> MQKIDEKLQLMNTIAKIYRGSIKEFNNRLGKLMNLSYLDFSILKATSEEPRSMVYLANRYFVTQSAITAAVDKLEAKGLVRRIRDSKDRRIVIVEITPKGRQV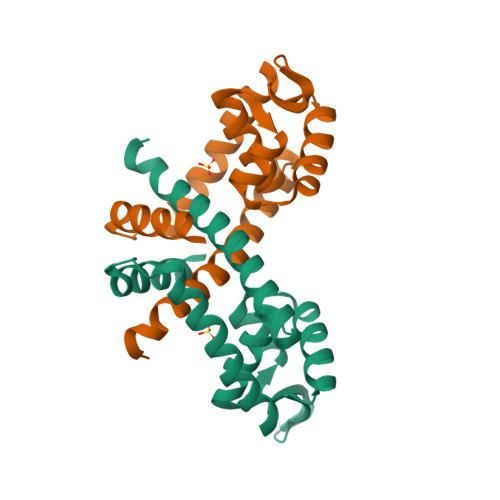LLEANEVLRNLVNEMLSDVENVEELLEGLNKILSRIGSSKD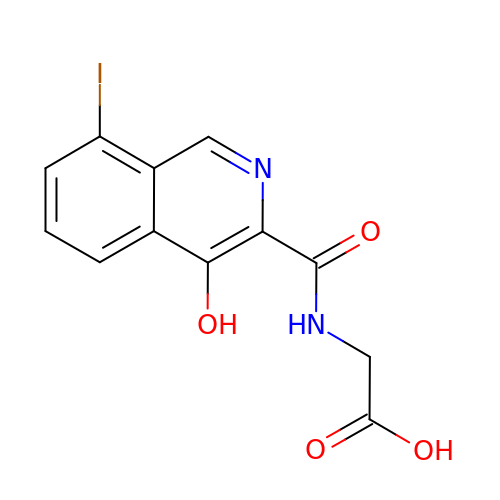N-[(4-HYDROXY-8-IODOISOQUINOLIN-3-YL)CARBONYL]GLYCINE | C12 H9 I N2 O4 | FUMNLXHPILGSLC-UHFFFAOYSA-N> MKTQVAIIGAGPSGLLLGQLLHKAGIDNVILERQTPDYVLGRIRAGVLEQGMVDLLREAGVDRRMARDGLVHEGVEIAFAGQRRRIDLKRLSGGKTVTVYGQTEVTRDLMEAREACGATTVYQAAEVRLHDLQGERPYVTFERDGERLRLDCDYIAGCDGFHGISRQSIPAERLKVFERVYPFGWLGLLADTPPVSHELIFANHPRGFALCSQRSATRSRYYVQVPLSEKVEDWSDERFWTELKARLPSEVAEKLVTGPSL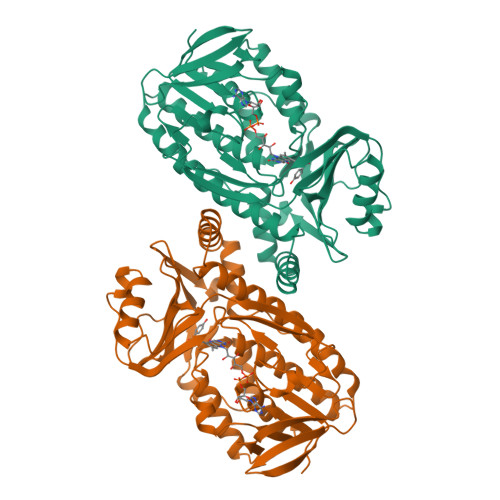EKSIAPLRSFVVEPMQHGRLFLAGDAAHIVPPTGAKGLNLAASDVSTLYRLLLKAYREGRGELLERYSAICLRRIWKAERFSWWMTSVLHRFPDTDAFSQRIQQTELEYYLGSEAGLATIAENYVGLPYEEIE>KLKQMIKNECEKDNQLAARLAKLAGYEKVNGFYKFVNTPEKEMENLGGLLKIVKNLFPDSEEQLLSEYFLELDPNKKCARQSVEYSDINQWDTLTDKIIINLCNSKNSTSQEWGKVYSLHRKLNKNEISLNDAIRESGKCKIKSAEMLFFSNAMLMYAYLNIGEFGLMKSTSKLLEFDDLPEGFIKESFKSRVSMLEANISLNENSLLEARQHSNRAIENSNVNRICFFAYLTIGNTLIFEDYDEAKKAYIKGQKYAKNPVHQEMLDGALCFLSNIWKKENQWVNYNSDNIKYLQLRAFYYINQGNIEEAT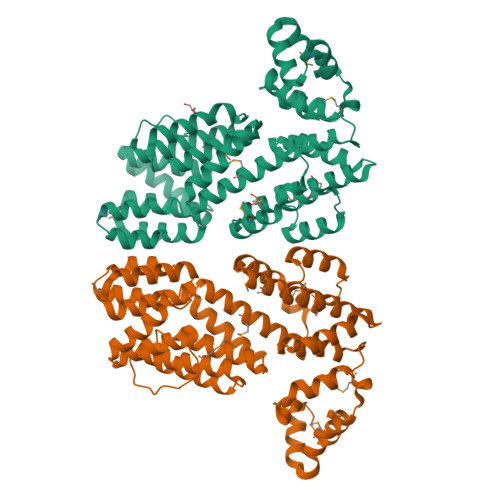EILDELSSRDQDENELGFYYYYKGLISQDKTDYYKSIRYFKKSDDKYFIQLPLLQLERMGADLELLNLISI[2x]>[2x]GSEKKLDALLAMPVKETKVFVESNEEPLFVMLKSSLSEETDETVGKPVVSEKTAEPGQDNDGETGGAWMQQLRHQADQGDAKSAFWLGRFTVEDSRDGKTIDEGIRLIRRSAEGGFVRAQLYLGTLYANGTHVKADPHEAEKWLSRAAGQGSPMVQLYLGLMYGHGKGVPRDLNKSLFWVEKAADRGLPHAQLARGLFASFSH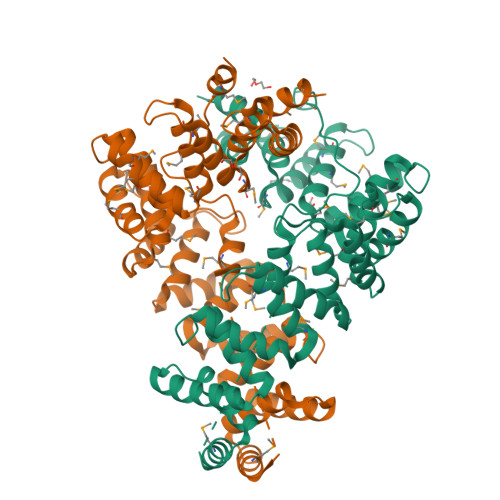YYPRDDEKAVLYLTKAAKQGMPMAQFYLALMYQRGRGVEQSNEQALHWNMLAAEQGYPDAEYAMSRMAELGIGVTADKAWSMMWLDRAAHHGMPLAQYLMGMAYLEGKSVPQDLPVAAAWFYKAAMQGNADAQLRLGYMYARGIGVPVDKPKAVAWLEKAASAGNTVAGQWLKQLD>[6x]PIELLPETPSQTAGPYVHIGLALEAAGNPTRDQEIWNRLAKPDAPGEHILLLGQVYDGNGHLVRDSFLEVWQADANGEYQDAYNLENAFNSFGRTATTFDAGEWTLHTVKPGVVNNAAG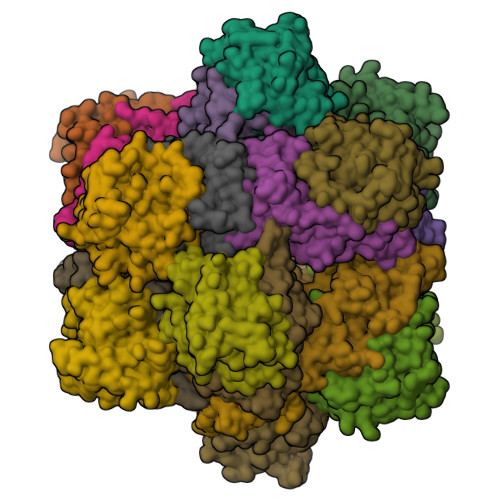VPMAPHINISLFARGINIHLHTRLYFDDEAQANAKCPVLNLIEQPQRRETLIAKRCEVDGKTAYRFDIRIQGEGETVFFDF;>PAQDNSRFVIRDRNWHPKALTPDYKTSIARSPRQALVSIPQSISETTGPNFSHLGFGAHDHDLLLNFNNGGLPIGERIIVAGRVVDQYGKPVPNTLVEMWQANAGGRHRHKNDRYLAPLDPNFGGVGRCLTDSDGYYSFRTIKPGPYPWRNGPNDWRPAHIHFGISGPSIATKLITQLYFEGDPLIPMCPIVKSIANPEAVQQLIAKLDMNNANPMDCLAYRFDIVLRGQRKTHFENC[6x]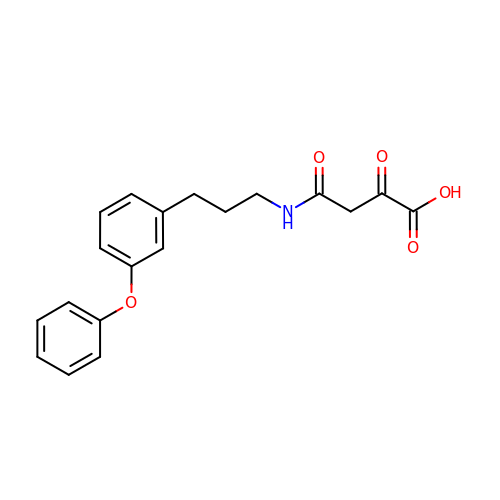2,4-dioxo-4-{[3-(3-phenoxyphenyl)propyl]amino}butanoic acid | C19 H19 N O5 | SJGQLSMZNBWNEL-UHFFFAOYSA-N> LKLCSPEEFTRLCREKTQEIYPIKEANGRTRKALIICNTEFKHLSLRYGANFDIIGMKGLLEDLGYDVVVKEELTAEGMESEMKDFAALSE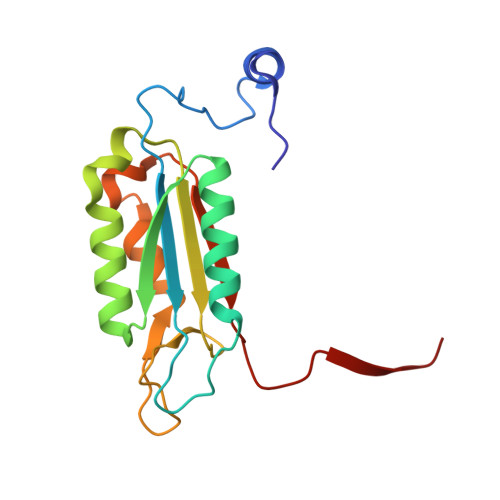HQTSDSTFLVLMSHGTLHGICGTMHSEKTPDVLQYDTIYQIFNNCHCPGLRDKPKVIIVQAARGGNSGEMWIRE>PKYRMSRPTCRGQKWTVMSNVWTSRWVATGTNARNIRPPTAIFLKKGLRAVSLAHNTAGPNPLSGTGSDRSEFRDLITWSPSGYPGDESTETICKAWSFFACFDGKEDLIGCISGPDNNAVLTIMYGGKPTDLYNSYALDILRTMESQCVCNNGTCSAMITDGPDIGPSKARMLFIKEGKIEKVVIVDGPGSSMVEECSCINEDSNEFGCLCRDNTANSRRPFLKCFWDSRTCKADYTCSQTLLDCPRPNDSIQTCGTSFGSLAGGLKGAYIPLGKGRICATRTVDKIQRKGMELMCTNGNILLEQDAMKKIGDLVTPTAQTGYSSATTIPRATEECDTICVATELVFSGAKGTNADLVIHC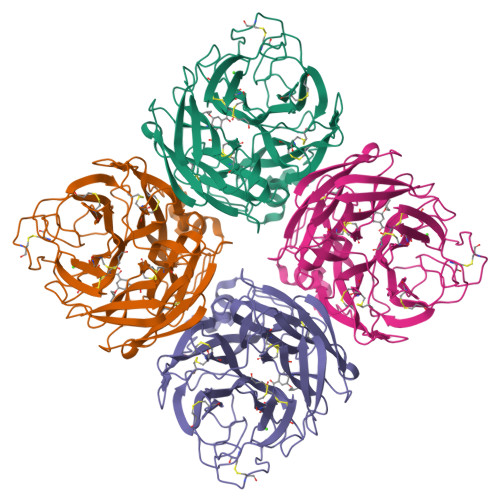LLGEARETESVVTAVVDRTTYSSLL[2x]(5Z)-3-(4-CHLOROPHENYL)-4-HYDROXY-5-(1-NAPHTHYLMETHYLENE)FURAN-2(5H)-ONE 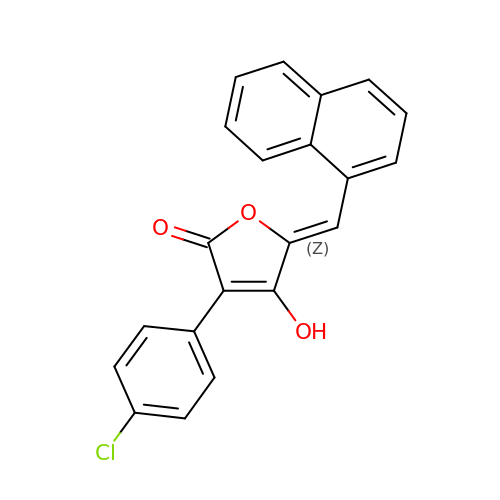| C21 H13 Cl O3 | PLGHLEBIWUQEPR-PDGQHHTCSA-N We previously designed adenosine-SAM bisubstrate analogues that contain the SAM cofactor with the S-atom replaced by a N-atom directly linked to an adenosine at the point of nucleophilic attack to mimic the substrate/cofactor bound state. These molecules were used to study the substrate recognition of the m6A MTase RlmJ, the Ribosomal RNA large subunit methyltransferase J that N6-methylates the adenine A2030 of the E. coli 23S rRNA. m6A RNA methyltransferases (MTases) catalyze the transfer of the methyl group from the cofactor S-adenosyl-L-methionine (SAM) to the N6-atom of adenines at specific positions in RNA, releasing the cofactor product S-adenosyl-l-homocysteine (SAH). Two crystal structures of RlmJ in complex with RNA–SAM conjugates were solved and revealed the RNA-specific recognition elements used by RlmJ to clamp the RNA substrate in its active site.

Crystals were obtained for GA* and GA*A bound to RlmJ at a RlmJ/ GA* ratio of 1/2 and RlmJ/GA*A ratio of 1/8. The GA*A conjugate density was not well-defined with RlmJ/GA*A ratios <1/8. The structures of RlmJ bound with GA* or GA*A were refined to 2.3 Å and 1.6 Å, respectively. In the RlmJ/GA*A structure, the ligand is folded via π-stacking of the ASAM moiety with the guanine moiety of GA*A. Compared to SAH, only the methionine part of CA is well-positioned in the active site of RlmJ. Asub is pushed out of the active site and unable to form the stabilising interactions with H9, N12, K18, and W195, observed for the GA* conjugate. The GA*A conjugate is maintained bound to RlmJ through correct binding of the methionine part and the stacking of the adenosine at the 3′-end (A3′ in Figure 5, corresponding to A2031 in the E. coli rRNA) with the conserved residue F8. A folded conformation was not found for the GA* conjugate, suggesting that the formation of such a folded conformation depends on the RNA length and sequence. F8 π-stacks with A3′ in the GA*A-bound RlmJ structure whereas H9 π-stacks with Asub in the GA*-bound RlmJ structure.

>[2x]MLSYRHSFHAGNHADVLKHTVQSLIIESLKEKDKPFLYLDTHAGAGRYQLGSEHAERTGEYLEGIARIWQQDDLPAELEAYINVVKHFNRSGQLRYYPGSPLIARQLLREQDSLQLTELHPSDYPLLRSEFQKDSRARVEKADGFQQLKAKLPPVSRRGLILIDPPYEMKTDYQAVVSGIAEGYKRFATGTYALWYPVVLRQQIKRMIHDLEATGIRKILQIELAVLPDSDRRGMTASGMIVINPPWKLEQQMNNVLPWLHSKLVPAGTGHATVSWIVPE> MKKTLLIAAALFTAVSPV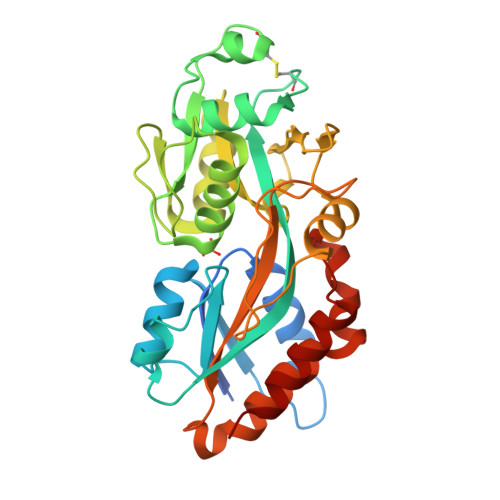MAGGRLSGAGASFPSKIYTRWFADLAKEKGAPRVNYQAVGSGSGRKAFIDETVNFGASDDPMKDKDIAKVKRGLVQIPMTGGTIAFGYNNPGCDLKLTQQKAVEVAMGQVTNWSELGCDDKKLTWAHRSDGSGTTKAFTNSMQAFSKTWTLGTGKSVAWPAGVGGKGNAGVAGVIRNTDGAIGYVNQSYIDENVRAAALQNLSGEFLKPSVEAGAKALNGITLDENLAGTNPNPTAKGAYPIATLTWILAYENGNGRNTKPVKTALSRLLSDEYQDKAPSLGFVPLKGDILEKARGAVERIGK Protective antigen (PA), the binding component of this AB toxin, forms an oligomeric pore that translocates lethal factor (LF) or edema factor, the active components of the toxin, into the cell. As the endosome acidifies, PAprepore undergoes a conformational change to a pore (PApore). This pore inserts into the endosomal membrane to form a channel. Three clamp sites aid in peptide translocation: the α clamp, the Φ clamp, and the charge clamp.

To prevent aggregation and migration of the nanodiscs to the air–water interface, we plunge froze the grids within 30 s of sample application. Using our TITaNS methodology, we obtained a 3.3 Å reconstruction of LFN translocating through PApore. Our reconstruction shows a loss of LFN density in the canonical binding site above the PApore. Notably, our reconstruction does not show density for residues 50–135 in the canonical folded LFN position. However, density for residues 136–250 are apparent. In addition to a loss of LFN density in the canonical binding site above the PApore, our reconstruction shows added density inside the pore lumen indicating a translocating complex. We attribute this density to unfolded LFN interacting with the benzyl rings of the PApore Φ clamp as LFN is translocating through the pore. In addition, the density for each of the PApore F427 residues was smeared in plane with the benzyl ring suggesting rotameric states moving up and down. Notably, density located at the PApore charge clamp is consistent with an α helix and suggests the deprotonated state of LF favors helix formation within the pore. Further down the pore we observe density for helix α1 emerging from the channel exit. Interestingly, the receptor binding domain did show different conformations for each protomer and indicates a degree of conformational flexibility.

>TVPDRDNDGIPDSLEVEGYTVDVKNKRTFLSPWISNIHEKKGLTKYKSSPEKWSTASDPYSDFEKVTGRIDKNVSPEARHPLVAAYPIVHVDMENIILSKNEDQSTQNTDSQTRTISKNTSTSRTHTSEVHGNAEVHASFFDIGGSVSAGFSNSNSSTVAIDHSLSLAGERTWAETMGLNTADTARLNANIRYVNTGTAPIYNVLPTTSLVLGKNQTLATIKAKENQLSQILAPNNYYPSKNLAPIALNAQDDFSSTPITMNYNQFLELEKTKQLRLDTDQVYGNIATYNFENGRVRVDTGSNWSEVLPQIQETTARIIFNGKDLNLVERRIAAVNPSDPLETTKPDMTLKEALKIAFGFNEPNGNLQYQGKDITEFDFNFDQQTSQNIKNQLAELNATNIYTVLDKIKLNAKMNILIRDKRFHYDRNNIAVGADESVVKEAHREVINSSTEGLLLNIDKDIRKILSGYIVEIEDTEGLKEVINDRYDMLNISSLRQDGKTFIDFKKYNDKLPLYISNPNYKVNVYAVTKENTIINPSENGDTSTNGIKKILIFSKKGYEIG[7x];> AGGHGDVGMHVKEKEKNKDENKRKDEERNKTQEEHLKEIMKHIVKIEVKGEEAVKKEAAEKLLEKVPSDVLEMYKAIGGKIYIVDGDITKHISLEALSEDKKKIKDIYGKDALLHEHYVYAKEGYCPVLVIQSSEDYVENTEKALNVYYEIGKILSRDILSKINQPYQKFLDVLNTIKNASDSDGQDLLFTNQLKEHPTDFSVEFLEQNSNEVQEVFAKAFAYYIEPQHRDVLQLYAPEAFNYMDKFNEQEINLSLEELKDQR> GGCUUCGCAAGA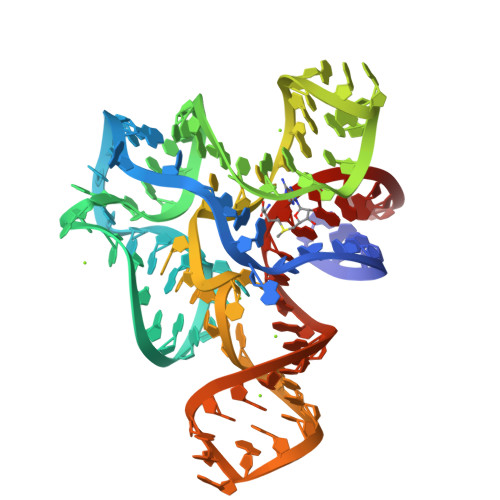GAGGUGGAGGGACUGGCCCGACGAAACCCGGCAACCAGAAAUGGUGCCAAUUCCUGCAGCGGAAACGUUGAAAGCGGAGCCG>[2x]FTGSEIFLASKRAAITYDTDPATGEPRAWLAPGGTGNVVAEQAGVLNISWIASADSEDDRRASALNPDGVTMELHSGREILVRLIRHDPAVFRNVQNFMTANLMWAANNYGWDRWTQPSFGSDAREGWADFGRFTRDFADAILKSSAQSADPVYLVHDYQLVGVPALLREQRPDAPILLFVHIPWPSADYWRILPKEIRTGILHGML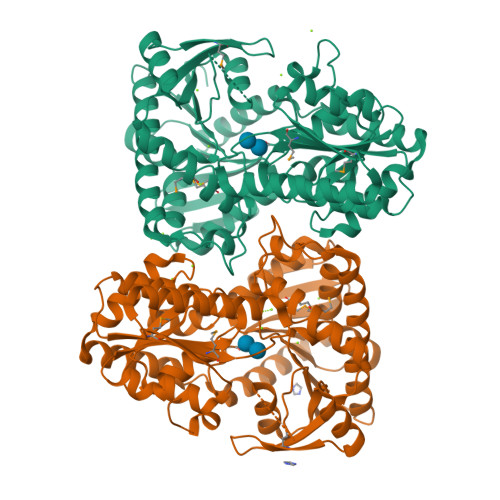PATTIGFFADRWCRNFLESVADLLPDARIDREAMTVEWRGHRTRLRTMPLGYSPLTLDGRNPQLPEGIEEWADGHRLVVHSGRTDPIKNAERAVRAFVLAARGGGLEKTRMLVRMNPNRLYVPANADYVHRVETAVAEANAELGSDTVRIDNDNDVNHTIACFRRADLLIFNSTVDGQNLSTFEAPLVNERDADVILSETCGAAEVLGEYCRSVNPFDLVEQAEAISAALAAGPRQRAEAAARRRDAARPWTLEAWVQAQLDGLAADHAARTATAERFDTAPAVSTRADL> GDE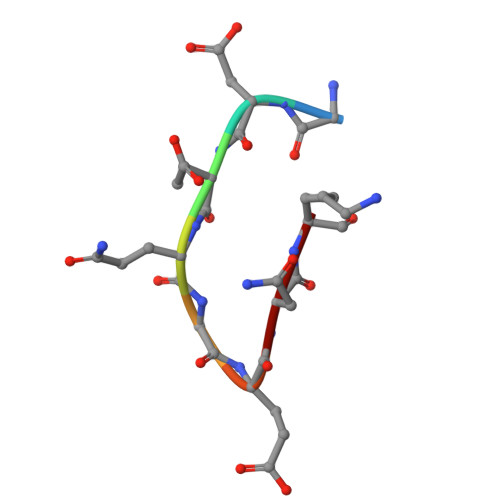QGENK>MKEFYLTVEQIGDSIFERYIDSNGRERTREVEYKPSLFAHCPESQATKYFDIYGKPCTRKLFANMRDASQWIKRMEDIGLEALGMDDFKLAYLSDTYNYEIKYDHTKIRVANFDIEVTSPDGFPEPSQAKHPIDAITHYDSIDDRFYVFDLLNSPYGNVEEWSIEIAAKLQEQGGDEVPSEIIDKIIYMPFDNEKELLMEYLNFWQQKTPVILTGWNVESFAIPYVYNRIKNIFGESTAKRLSPHRKTRVKVIENMYGSREIITLFGISVLDYIDLYKKFSFTNQPSYSLDYISEFELNVGKLKYDGPISKLRESNHQRYISYNIIAVYRVLQIDAKRQFINLSLDMGYYAKIQIQSVFSPIKTWDAIIFNSLKEQNKVIPQGRSHPVQPYPGAFVKEPIPNRYKYVMSFDLTSLYPSIIRQVNISPETIAGTFKVAPLHDYINAVAERPSDVYSCSPNGMMYYKDRDGVVPTEITKVFNQRKEHKGYMLAAQRNGEIIKEALHNPNLSVDEPLDVDYRFDFSDEIKEKIKKLSAKSLNEMLFRAQRTEVAGMTAQINRKLLINSLYGALGNVWFRYYDLRNATAITTFGQMALQWIERKVNEYLNEVCGTEGEAFVLYGDTDSIYVSADKIIDKVGESKFRDTNHWVDFLDKFARERMEPAIDRGFREMCEYMNNKQHLMFMDREAIAGPPLGSKGIGGFWTGKKRYALNVWDMEGTRYAEPKLKIMGLETQKSSTPKAVQKALKECIRRMLQEGEESLQEYFKEFE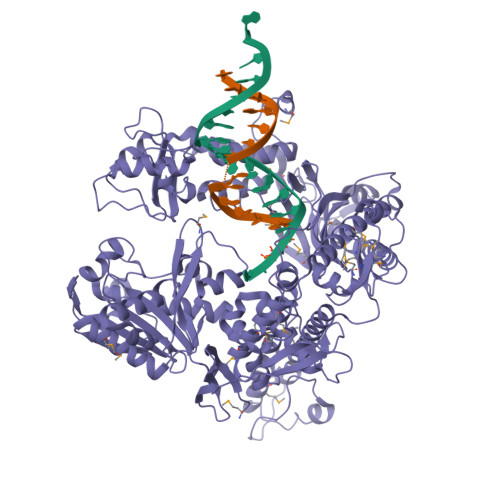KEFRQLNYISIASVSSANNIAKYDVGGFPGPKCPFHIRGILTYNRAIKGNIDAPQVVEGEKVYVLPLREGNPFGDKCIAWPSGTEITDLIKDDVLHWMDYTVLLEKTFIKPLEGFTSAAKLDYEKKASLFDMFDF[4x]> GPLGSMSQSNRELVVDFLSYKLSQKGYSWSQMAAVKQALREAGDEFELRYRRAFSDLTSQLHITPGTAYQSFEQVVNELFRDGVNWGRIVAFFSFGGALCVESVDKEMQVLVSRIAAWMATYLNDHLEPWIQENGGWDTFVELYGNNAAAESRKGQER;> LPLEPNSILGQVGR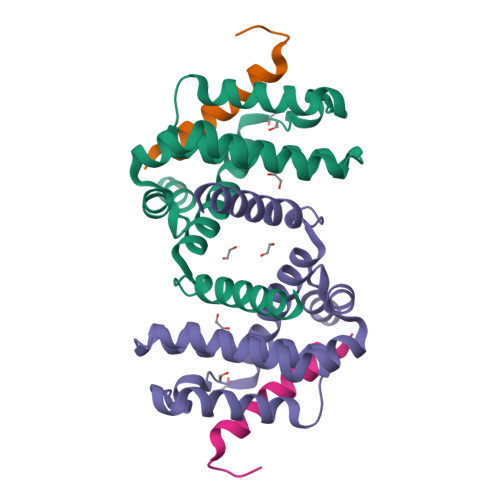LLALIGDDINRRYDTEFQNL> DPMKNTCKLLVVADHRFYRYMGRGEESTTTNYLIELIDRVDDIYRNTAWDNAGFKGYGIQIEQIRILKSPQEVKPGEKHYNMAKSYPNEEKDAWDVKMLLEQFSFDIAEEASKVCLAHLFTYQDFDMGTLGLAYVGSPRANSHGGVCPKAYYSPVGKKNIYLNSGLTSTKNYGK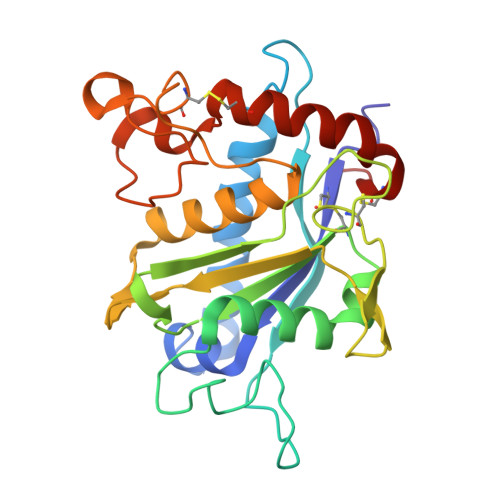TILTKEADLVTTHELGHNFGAEHDPDGLAECAPNEDQGGKYVMYPIAVSGDHENNKMFSQCSKQSIYKTIESKAQECFQERS> MGSSHHHHHHSSGLVPAGSHMTSINPIFEPFIEAHRYKVAKGGRGSGKSWAIARLLVEAARRQPVRILCARELQNSISDSVIRLLEDTIEREGYSAEFEIQRSMIRHLGTNAEFMFYGIKNNPTKIKSLEGIDICWVEEAEAVTKESWDILIPTIRKPFSEIWVSFNPKNILDDTYQRFVVNPPDDICLLTVNYTDNPHFPEVLRLEMEECKRRNPTLYRHIWLGEPVSASDMAIIKREWLEAATDAHKKLGWKAKGAVVSAHDPSDTGPDAKGYASRHGSVVKRIAEGLLMDINEGADWATSLAIEDGADHYLWDGDGVGAGLRRQTTEAFSGKKIT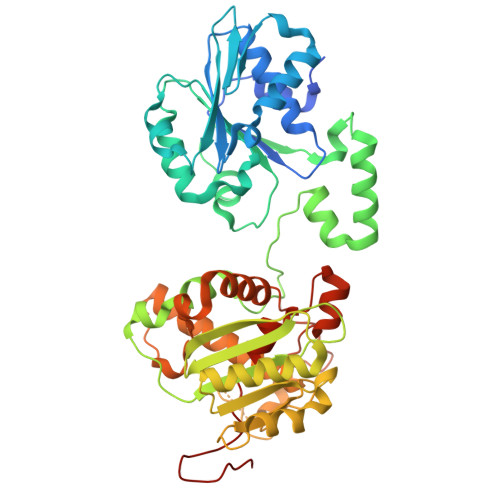ATMFKGSESPFDEDAPYQAGAWADEVVQGDNVRTIGDVFRNKRAQFYYALADRLYLTYRAVVHGEYADPDDMLSFDKEAIGEKMLEKLFAELTQIQRKFNNNGKLELMTKVEMKQKLGIPSPNLADALMMCMHCPALVREETEIYVPSSSGW> NRLFR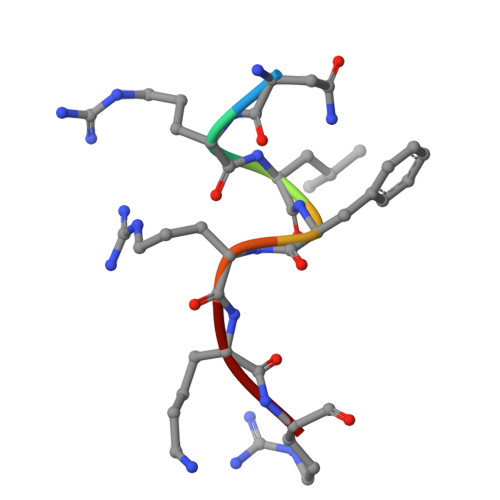KR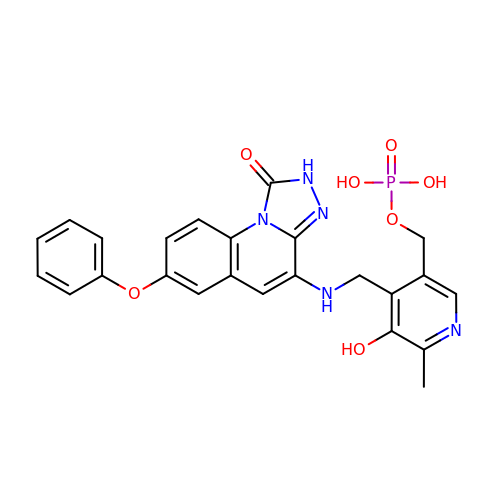(5-hydroxy-6-methyl-4-{[(1-oxo-7-phenoxy-1,2-dihydro[1,2,4]triazolo[4,3-a]quinolin-4-yl)amino]methyl}pyridin-3-yl)methyl dihydrogen phosphate | C24 H22 N5 O7 P | AMDYNPYMOMDDSQ-UHFFFAOYSA-N> IVGGQECKDGECPWQALLINEENEGFCGGTILSEFYILTAAHCLYQAKRFKVRVGDRNTEQEEGGEAVHEVEVVIKHNRFTKETYDFDIAVLRLKTPITFRMNVAPACLPERDWAESTLMTQKTGIVSGFGRTHE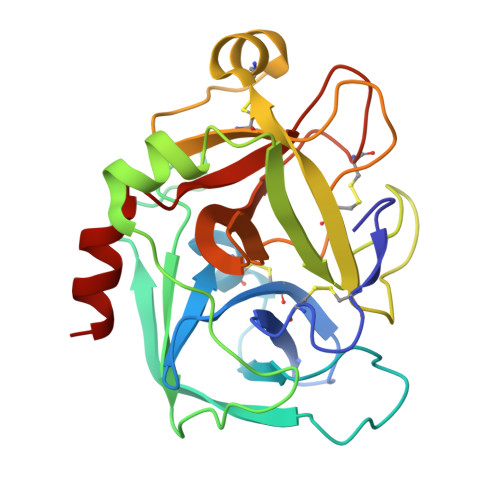KGRQSTRLKMLEVPYVDRNSCKLSSSFIITQNMFCAGYDTKQEDACQGDSGGPHVTRFKDTYFVTGIVSWGEGCARKGKYGIYTKVTAFLKWIDRSMK> GSHMFDYMFKILIIGNSSVGKTSFLFRYADDSF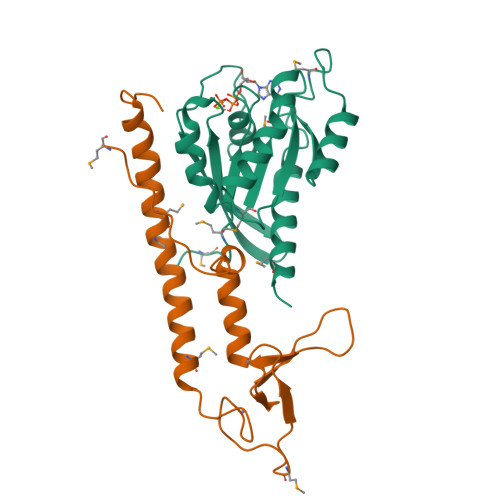TPAFVSTVGIDFKVKTIYRNDKRIKLQIWDTAGLERYRTITTAYYRGAMGFILMYDITNEESFNAVQDWSTQIKTYSWDNAQVLLVGNKCDMEDERVVSSERGRQLADHLGFEFFEASAKDNINVKQTFERLVDVICEKMSESLDTADPAVTGAKQGPQLTDQQAPPHQD;> GSHMRKQEELTDEEKEIINRVIARAEKMETMEQERIGRLVDRLETMRKNVAGDGVNRCILCGEQLGMLGSASVVCEDCKKNVCTKCGVETSNNRPHPVWLCKICLEQREVWKRSGAWFFKGFPKQVLPQPMPIK>MGHHHHHHHHHHHHSSGHIDDDDKHMLEMIQSHPLLAAPLAVGDTIGFFSSSAPATVTAKNRFFRGVEFLQRKGFKLVSGKLTGKTDFYRSGTIKERAQEFNELVYNPDITCIMSTIGGDNSNSLLPFLDYDAIIANPKIIIGYADTTALLAGIYAKTGLITFYGPALIPSFGEHPPLVDITYESFIKILTRKQSGIYTYTLPEKWSDESINWNE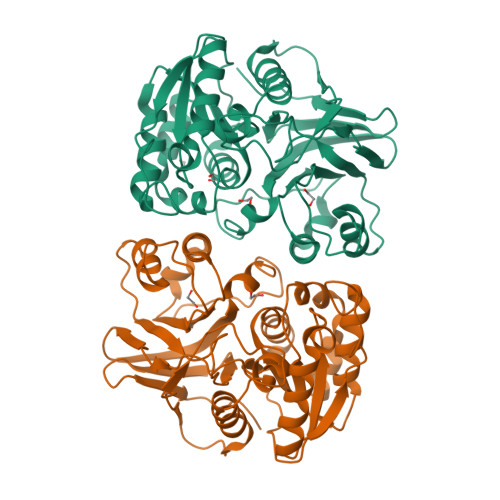NKILRPKKLYKNNCAFYGSGKVEGRVIGGNLATLTGIWGSEWMPEIRNGDILFIEDSRASIATVERLFSMLKLNRVFDKVSAIILGKHELFDCAGSKRRPYEVLTEVLDGKQIPVLDGFDCSHTHPMLTLPLGVKLAIDFDNKNISITEQYLSTEK[2x]>MSLRPLYMDVQATTPLDPRVLDAMLPYLINYYGNPHSRTHAYGWESEAAMERARQQVASLIGADPREIIFTSGATESNNIAIKGVARFYRSRKKHLITTQTEHKCVLDSCRSLEAEGFQVTYLPVQKSGIIDLKELEAAIQPDTSLVSVMTVNNEIGVKQPIAEIGRICSSRKVYFHTDAAQAVGKIPLDVNDMKIDLMSISGHKIYGPKGVGAIYIRRRPRVRVEALQSGGGQERGMRSGTVPTPLVVGLGAACEVAQQEMEYDHKRISKLSERLIQNIMKSLPDVVMNGDPKHHYPGCINLSFAYVEGESLLMALKDVALSSGSACTSASLEPSYVLRAIGTDEDLAHSSIRFGIGRFTTEEEVDYTVEKCIQHVKRLREMSPLWEMVQDGIDLKSIKWTQH[2x];>[2x]MGSSHHHHHHGSPTTENLYFQGHNMAASSRAQVLALYRAMLRESKRFSAYNYRTYAVRRIRDAFRENKNVKDPVEIQTLVNKAKRDLGVIRRQVHIGQLYSTDKLIIENRDMPRT;>[2x]MSTIEERVKKIIGEQLGVKQEEVTNNASFVEDLGADSLDTVELVMALEEEFDTEIPDEEAEKITTVQAAIDYINGHQA;>MAYHKKVVDHYENPRNVGSLDKTSKNVGTGLVGAPACGDVMKLQIQVDEKGKIVDARFKTFGCGSAIASSSLATEWVKGKTVEEALTIKNTDIAKELCLPPVKLHCSMLAEDAIKAALADYKLKQEPKKGEAEKKLEHHHHHH[2x];> MASDVVNVVFVDRSGQRIPVSGRVGDNVLHLAQRHGVDLEGACEASLACSTCHVYVSEDHLDLLPPPEEREDDMLDMAPLLQENSRLGCQIVLTPELEGAEFTLPKITRNFYVDGHVPKPH

The process is initiated by the mitochondrial core ISC complex, which synthesizes a [2Fe-2S] cluster de novo from cysteine-derived sulfur and ferrous iron (Fe2+). This complex is composed of the iron-sulfur scaffold protein ISCU2, the dimeric pyridoxal phosphate (PLP)-dependent cysteine desulfurase subcomplex NFS1-ISD11-ACP1, the allosteric regulator frataxin (FXN), and the electron donor ferredoxin-2 (FDX2), which is itself reduced by the NADPH-dependent ferredoxin reductase (FDXR). The sulfane sulfur (S0) of the persulfide on ISCU2 is reduced to sulfide (S2-) by FDX2 to initiate [2Fe-2S] cluster formation. FDX2 and FXN compete for binding to overlapping sites at the core ISC complex during de novo [2Fe-2S] cluster biosynthesis.

First, to elucidate the interaction site of reduced FDX2 with the (NIAU)2 complex, the (NIA)2 subcomplex was incubated for 20 min with iron-loaded ISCU2 and FDXR-reduced FDX2 to yield the (NIAUF)2 sample. In the (NIAUF)2 dataset, 61% of the particles belong to a class in which FDX2 is bound in the proximal conformation, and 39% belong to a distal-bound FDX2 class. Additional weak density at this site, typically associated with conformational and/or compositional heterogeneity in cryo-EM, was further assessed by C2 symmetry expansion and focused 3D classification. This revealed two major FDX2 conformations that we refer to as ‘proximal’ and ‘distal’ according to the distances between the [2Fe-2S] cluster of FDX2 and the FeS cluster assembly site of ISCU2, namely 23 Å for the distal conformation and 14 Å for the proximal conformation. In the distal conformation, fewer salt bridges are formed with NFS1’ than in the proximal conformation and the overall resolution of FDX2 is lower than for the rest of the complex, indicating a more flexible binding mode in the distal position than in the proximal conformation, where FDX2 appears well resolved. In the distal binding position, the C-terminal 15 residues of FDX2 are unresolved, indicating that these residues are highly flexible when FDX2 is bound in this conformation. In the distal conformation, the [2Fe-2S] cluster of FDX2 is too far for efficient electron transfer to the ISCU2 FeS cluster assembly site (23 Å), whereas the movement to the proximal binding position brings the [2Fe-2S] cluster to a distance of 14 Å that would allow rapid electron transfer for reduction of the Cys138ISCU2 persulfide. A possible explanation for the existence of two binding modes for FDX2 could be that the distal conformation is kinetically favored and represents a first stage of binding, which then enables the intrinsically disordered C terminus of FDX2 to rigidify and transiently bind to NFS1. (5.1) Reduced FDX2 binds loosely to the NFS1 arginine patch in the distal conformation.> NHPMLMNLL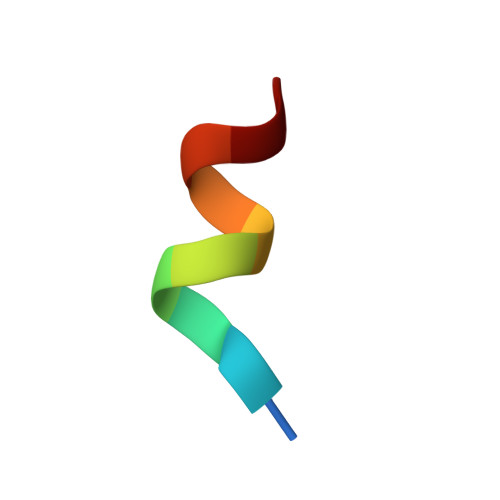K>MAKKTSSKGKLPPLAPGFLHLLQPDLPIYLLGLTQKFGPIYRLHLGLQDVVVLNSKRTIEEAMVKKWADFAGRPEPLTYKLVSRNYPDLSLGDYSLLWKAHKKLTRSALLLGIRDSMEPVVEQLTQEFCERMRAQPGTPVAIEEEFSLLTCSIICYLTFGDKIKDDNLMPAYYKCIQEVLKTWSHWSIQIVDVIPFLRFFPNPGLRRLKQAIEKRDHIVEMQLRQHKESLVAGQWRDMMDYMLQGVAQPSMEEGSGQLLEGHVHMAAVDLLIGGTETTANTLSWAVVFLLHH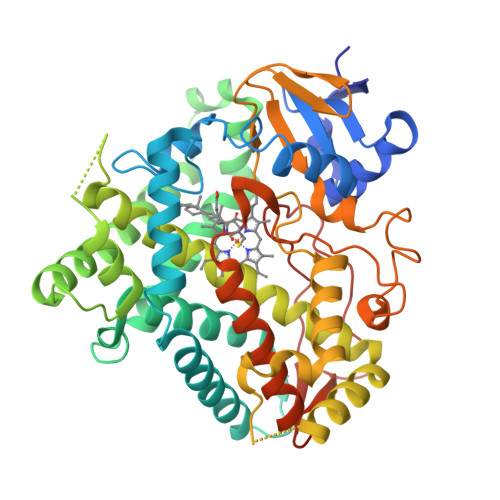PEIQQRLQEELDHELGPGASSSRVPYKDRARLPLLNATIAEVLRLRPVVPLALPHRTTRPSSISGYDIPEGTVIIPNLQGAHLDETVWERPHEFWPDRFLEPGKNSRALAFGCGARVCLGEPLARLELFVVLTRLLQAFTLLPSGDALPSLQPLPHCSVILKMQPFQVRLQPRGMGAHSPGQSQ[3x]PANTOTHENOIC ACID 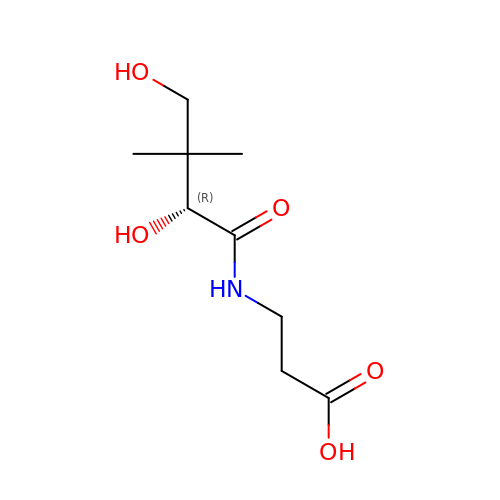| C9 H17 N O5 | GHOKWGTUZJEAQD-ZETCQYMHSA-N> WKWWEEERYPEGIKWKFLEHKGPVFAPPYEPLPENVKFYYDGKVMKLSPKAEEVATFFAKMLDHEYTTKEIFRKNFFKDWRKEMTNEEKNIITNLSKCDFTQMSQYFKAQTEARKQMSKEEKLKIKEENEKLLKEYGFCIMDNHKERIANFKIEPPGLFRGRGNHPKMGMLKRRIMPEDIIINCSKDAKVPSPPPGHKWKEVRHDNKVTWLVSWTENIQGSIKYIMLNPSSRIKGEKDWQKYETARRLKKCVDKIRNQYREDWKSKEMKV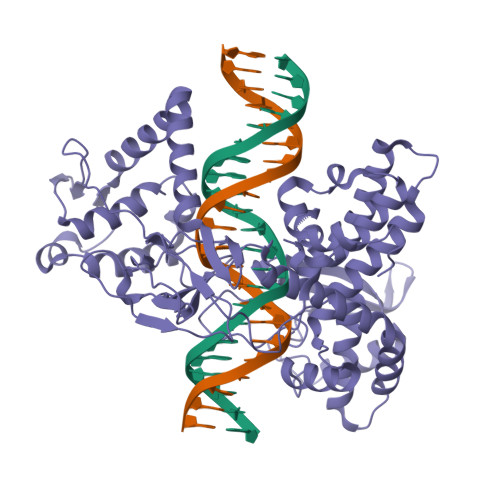RQRAVALYFIDKLALRAGNEKEEGETADTVGCCSLRVEHINLHPELDGQEYVVEFDFLGKDSIRYYNKVPVEKRVFKNLQLFMENKQPEDDLFDRLNTGILNKHLQDLMEGLTAKVFRTYNASITLQQQLKELTAPDENIPAKILSYNRANRAVAILCNHQIAPPKTFEKSMMNLQTKIDAKKEQLADARRDLKSAKADAKVMKDAKTKKVVESKKKAVQRLEEQLMKLEVQATDREENKQIALGTSKLNFLDPRITVAWCKKWGVPIEKIYNKTQREKFAWAIDMADEDYEF> MNIKKFAKQATVLTFTTALLAGGATQAFAKETNQKPYKETYGISHITRHDMLQIPEQQKNEKYQVPEFDSSTIKNISSAKGLDVWDSWPLQNADGTVANYHGYHIVFALAGDPKNADDTSIYMFYQKVGETSIDSWKNAGRVFKDSDKFDANDSILKDQTQEWSGSATFTSDGKIRLFYTDFSGKHYGKQTLTTAQVNVSASDSSLNINGVEDYKSIFDGDGKTYQNVQQFIDEGNYSSGDNHTLRAPHYVEDKGHKYLVFEANTGTEDGYQGEESLFNKAYYGKSTSFFRQESQKLLQSDKKRTAELANGALGMIELNDDYTLKKVMKPLIASNTVTDEI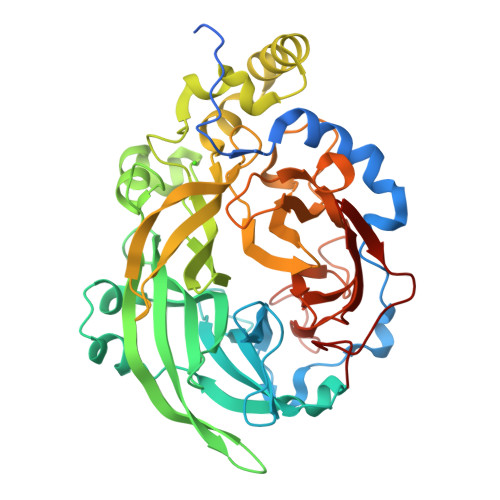ERANVFKMNGKWYLFTDSRGSKMTIDGITSNDIYMLGYVSNSLTGPYKPLNKTGLVLKMDLDPNDVTFTYSHFAVPQAKGNNVVITSYMTNRGFYADKQSTFAPSFLLNIKGKKTSVVKDSILEQGQLTVNK>[24x]MAIEIKVPDIGADEVEITEILVKVGDKVEAEQSLITVEGDKASMEVPSPQAGIVKEIKVSVGDKTQTGALIMIFDSADGAADAAPAQAEEKKEAAPAAAPAAAAAKDVNVPDIGSDEVEVTEILVKVGDKVEAEQSLITVEGDKASMEVPAPFAGTVKEIKVNVGDKVSTGSLIMVFEVAGEAGAAAPAAKQEAAPAAAPAPAAGVKEVNVPDIGGDEVEVTEVMVKVGDKVAAEQSLITVEGDKASMEVPAPFAGVVKELKVNVGDKVKTGSLIMIFEVEGAAPAAAPAKQEAAAPAPAAKAEAPAAAPAAKAEGKSEFAENDAYVHATPLIRRLAREFGVNLAKVKGTGRKGRILREDVQAYVKEAIKRAEAAPAATGGGIPGMLPWPKVDFSKFGEIEEVELGRIQKISGANLSRNWVMIPHVTHFDKTDITELEAFRKQQNEEAAKRKLDVKITPVVFIMKAVAAALEQMPRFNSSLSEDGQRLTLKKYINIGVAVDTPNGLVVPVFKDVNKKGIIELSRELMTISKKARDGKLTAGEMQGGCFTISSIGGLGTTHFAPIVNAPEVAILGVSKSAMEPVWNGKEFVPRLMLPISLSFDHRVIDGADGARFITIINNTLSDIRRLVM

The pyruvate dehydrogenase complex (PDHc) links glycolysis to the citric acid cycle by converting pyruvate into acetyl-coenzyme A. PDHc encompasses three enzymatically active subunits, namely pyruvate dehydrogenase, dihydrolipoyl transacetylase, and dihydrolipoyl dehydrogenase. Dihydrolipoyl transacetylase is a multidomain protein comprising a varying number of lipoyl domains, a peripheral subunit-binding domain, and a catalytic domain. It forms the structural core of the complex, provides binding sites for the other enzymes, and shuffles reaction intermediates between the active sites through covalently bound lipoyl domains. In Gram-negative bacteria the E2p catalytic domains are arranged in eight tight trimers further associated into a 24-meric cubic structure with an E2p trimer in each corner of the cube with a 432 symmetry.

We report here the cryo-EM reconstruction of the cubic E2p core of E. coli PDHc in a native resting state (in the absence of substrates), in which a lipoyl domain is bound to the catalytic domain of each E2p and the dihydrolipoyllysine residue is immerged deep in the E2p active site channel (coenzyme A is not present). We determined the cryo-EM structure of the cubic E2p core to a nominal resolution of 3.16 Å (FSC criterion of 0.143). The overall structure of the E2p shows the expected cubic core, consisting of trimers of the catalytic domains with the associated lipoyl domains, which bind to the catalytic domains in a manner that follows the overall octahedral symmetry of the entire complex. The interface area is 840 Å2, includes 24 pairs of interfacing residues, and is stabilized mostly by hydrophobic interactions, but also by polar interactions including hydrogen bonds and salt bridges. The lipoyl domain interacts with the catalytic domain through a striking electrostatic network. The lipoyl domain exhibits a large acidic patch that interacts with the positive dipole of the N-terminus of the catalytic domain helix H1 as well as with an arginine residue (R407) on the N-terminal tip of this helix. Specifically, two loops (residues 213–215 and 242–249) of the lipoyl domain form several hydrogen bonds with a loop of the catalytic domain (residues 536–544) located along the entrance into the active channel, and there is also a van der Waals interaction between methionine M248 from the lipoyl domain and methionine M543 from the catalytic domain. The dihydrolipoyllysine (K245) itself forms predominantly hydrophobic interactions with residues of the channel leading into the catalytic site, which is formed at the interface between two catalytic domains, and both thiol groups are engaged in polar interactions. In our structure the reactive terminal sulfur (S8) of the dihydrolipoamide, which normally carries the acetyl group, is oriented towards a nitrogen atom (NE2) of the catalytic histidine H603′ and is in a close proximity to S551 and D607′.> GTVLAEDQLAQMSKQLDMFKTNL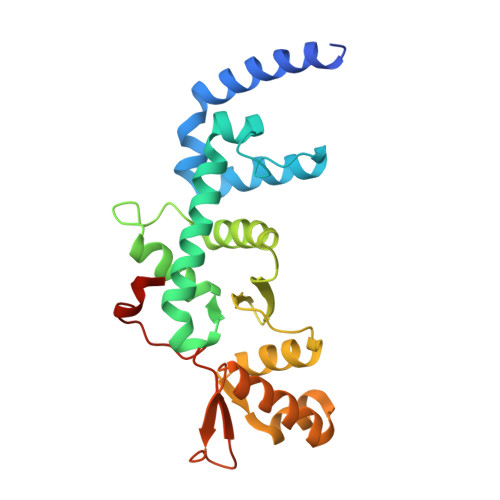EEFASKHKQEIRKNPEFRVQFQDMCATIGVDPLASGKGFWSEMLGVGDFYYELGVQIIEVCLALKHRNGGLITLEELHQQVLKGRGKFAQDVSQDDLIRAIKKLKALGTGFGIIPVGGTYLIQSVPAELNMDHTVVLQLAEKNGYVTVSEIKASLKWETERARQVLEHLLKEGLAWLDLQAPGEAHYWLPALFTDLYSQEITAEEAREALP>[2x]MGSSHHHHHHSSGRENLYFQGVQHTIAR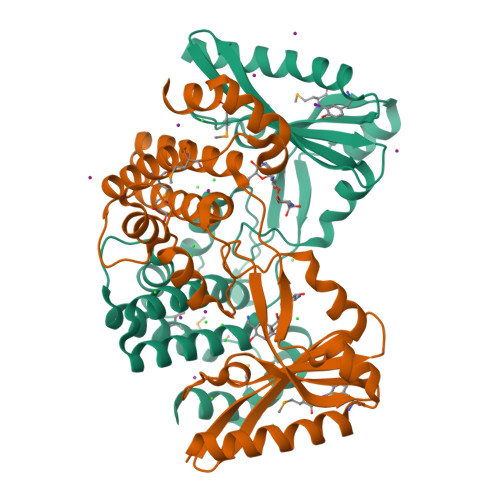WVDRLREEYADAVAILLKGSYARGDAATWSDIDFDVLVSTQDVEDYRTWIEPVGDRLVHISAAVEWVTGWERDTVDPSSWSYGLPTQETTRLMWAINDETRRRLDRPYKTHPAAEPEVEDTVEALGKIRNAIARGDDLGVYQSAQTVAKLVPTLLIPINPPVTVSHARQAIEAILAFPRVPVGFAADWLTCLGLVEERSARSTAAAAERMVRGVLEMLPTDPDLLGEDIARLMNAGLLEKYVQQ> GSSEGTSCNSIVNGCPNLDFNWHMDQQNIMQYTLDVTSVSWVQDNTYQITIHVKGKENIDLKYLWSLKII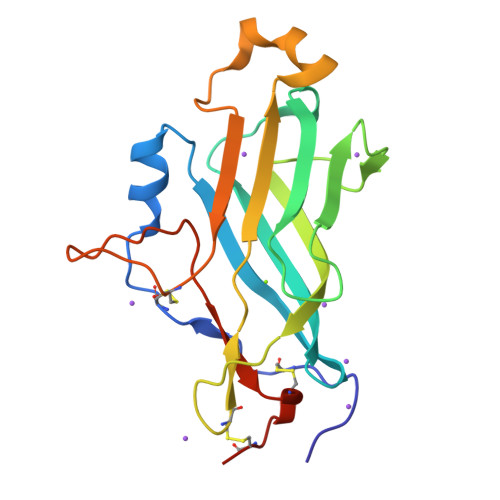GVTGPKGTVQLYGYNENTYLIDNPTDFTATFEVYATQDVNSCQVWMPNFQIQFEYLQGSAAQYASSWQWGTTSFDLSTGCNNYDNQGHSQTDFPGFYWNIDCDNNCGGTKSS> MLGHLVGLVKVRVVRGVNLAVRDLRSSDPYVIVRMGKQKLKTRVIKKTT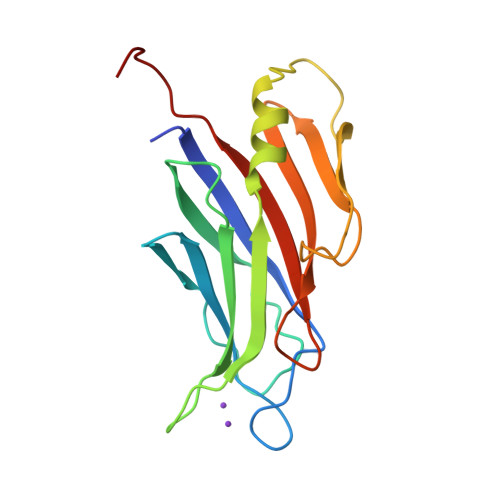NPEWNDELTLSIEDPAVPVRLEVYDKDTFIDDAMGNAELDIRPLVEVVKMKIEGVADNTVVKKVVPNRQNCLAEESTIYISEGKVKQDVVLRLRDVECGEIELQLQWVDIPGSKGV>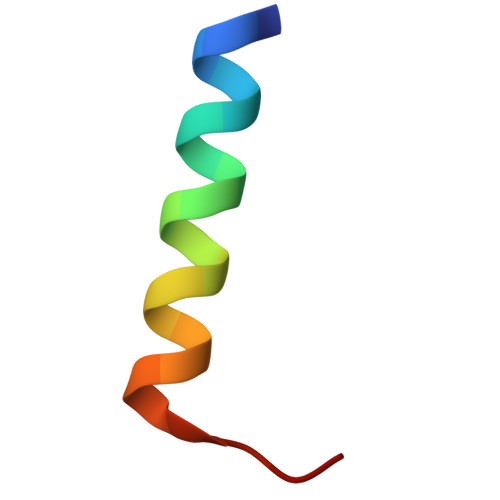 LFLLTVCTTVLVSGWVVLGWME asciminib | C20 H18 Cl F2 N5 O3 | 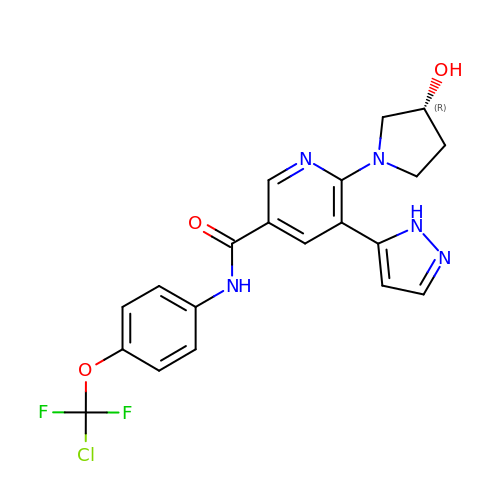VOVZXURTCKPRDQ-CQSZACIVSA-N>[2x]GPGYQDPNSAKLLQILNVRVVGSGERVVVLSHGFGTDQSAWSRVLPYLTRDHRVVLYDLVCAGSVNPDHFDFRRYDNLDAYVDDLLAILDALRIPRCAFVGHSVSAMIGILASIRRPDLFAKLVLIGASPRFLNDSDYHGGFELEEIQQVFDAMGANYSAWATGYAPLAVGADVPAAVQEFSRTLFNMRPDISLHVCQTVFKTDLRGVLGMVRAPCVVVQTTRDVSVPA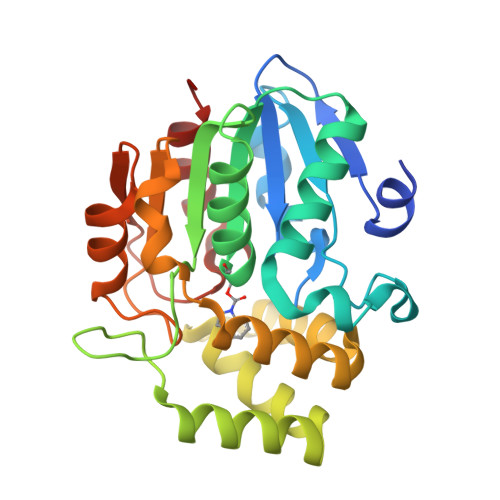SVAAYLKAHLGGRTTVEFLQTEGHLPHLSAPSLLAQVLRRALARY> MVANPEHYIKHPLQNRWALWFFKNDKSKTWQANLRLISKFDTVEDFWALYNHIQLSSNLMPGCDYSLFKDGIEPMWEDEKNKRGGRWLITLNKQQRRSDLDRFWLETLLCLIGESFDDYSDDVCGAVVNVRAKGDKIAIWTTECENREAVTHIGRVYKERLGLPPKIVIG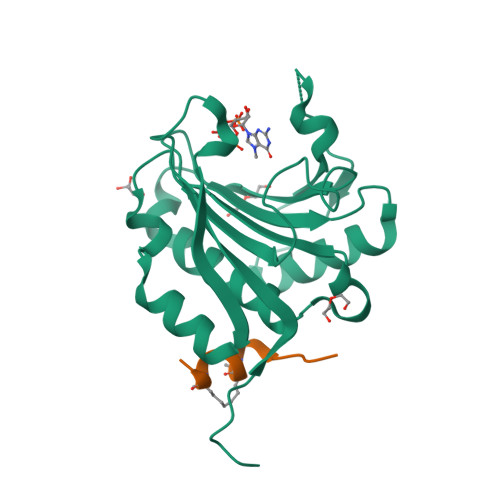YQSHADTATKSGSTTKNRFVV;> XRIIYSRLQLLLLKX>[30x]MSDGAVQP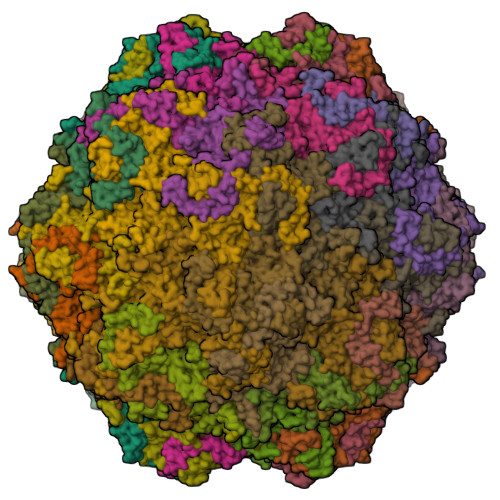DGGQPAVRNERATGSGNGSGGGGGGGSGGVGISTGTFNNQTEFKFLENGWVYITANSSRLVHLNMPESENYRRVVVNNLDKTAVNGNMALDDTHAEIVTPWSLVDANAWGVWFNPGDWQLIVNTMSELHLVSFEQEIFNVVLKTVSESATQPPTKVYNNDLTASLMVALDSNNTMPFTPAAMRSETLGFYPWKPTIPTPWRYYFQWDRTLIPSHTGTSGTPTNIYHGTDPDDVQFYTIENSVPVHLLRTGDEFATGTFFFDCKPCRLTHTWQTNRALGLPPFLNSLPQSEGGTNFGYIGVQQDKRRGVTQMGNTNYITEATIMRPAEVGYSAPYYSFEASTQGPFKTPIAAGRGGAQTDENQAADGDPRYAFGRQHGQKTTTTGETPERFTYIAHQDTGRYPEGDWIQNINFNLPVTDDNVLLPTDPIGGKTGINYTNIFNTYGPLTALNNVPPVYPNGQIWDKEFDTDLKPRLHVNAPFVCQNNCPGQLFVKVAPNLTNQYDPDASANMSRIVTYSDFWWKGKLVFKAKLRASHTWNPIQQMSINVDNQFNYVPSNIGGMKIVYEKSQLAPRKLY> GCGGAAGUAGUUCAGUGGUAGAACACCGGGUGGAACCCCAGGAAACUGGCCCGGGUCGCGCGG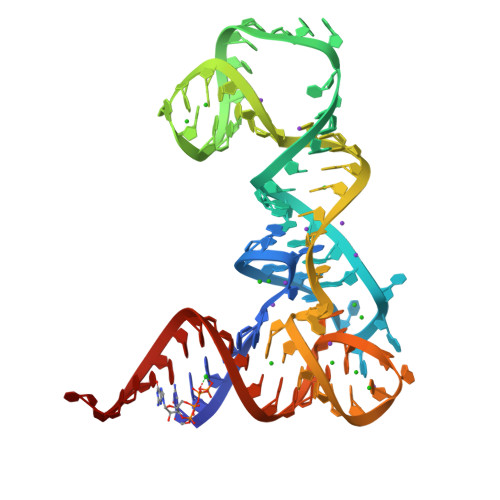GUUCGAGUCCCGUCUUCCGCUCC>GPNADINLEESIRESLQKRELLKSQVEDFTRIFLPIYDSLMSSQNKLFYITNADDSTKFQLVNDVMDELITSSARKELPIFDYIHIDALELAGMDALYEKIWFAISKENLCGDISLEALNFYITNVPKAKKRKTLILIQNPENLLSEKILQYFEKWISSKNSKLSIICVGGHNVTIREQINIMPSLKAHFTEIKLNKVDKNELQQMIITRLKSLLKPFHVKVNDKKEMTIYNNIREGQNQKIPDNVIVINHKINNKITQLIAKNVANVSGSTEKAFKICEAAVEISKKDFVRKGGLQK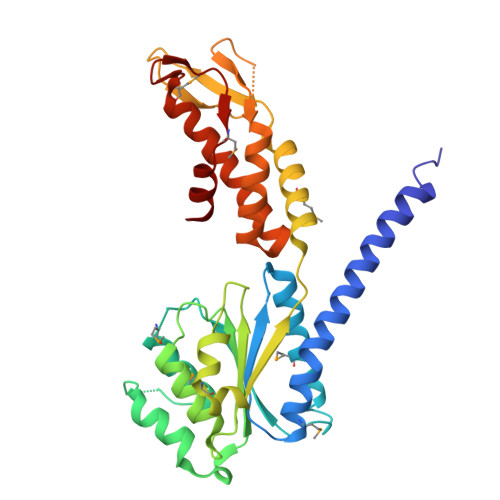GKLVVSQEMVPRYFSEAING[2x]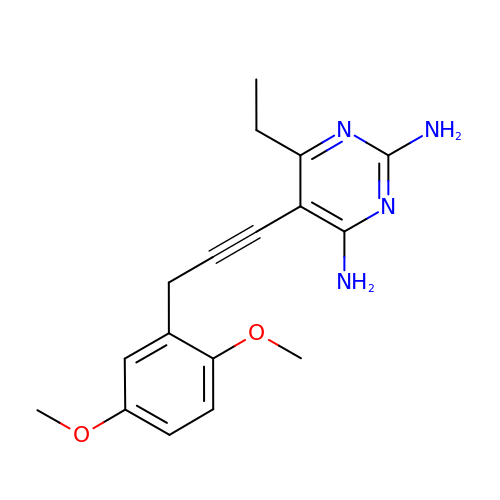5-[3-(2,5-dimethoxyphenyl)prop-1-yn-1-yl]-6-ethylpyrimidine-2,4-diamine | C17 H20 N4 O2 | NNFDQABYXZBKRK-UHFFFAOYSA-N>MIPARFAGVLLALALILPGTLCAEGTRGRSSTARCSLFGSDFVNTFDGSMYSFAGYCSYLLAGGCQKRSFSIIGDFQNGKRVSLSVYLGEFFDIHLFVNGTVTQGDQRVSMPYASKGLYLETEAGYYKLSGEAYGFVARIDGSGNFQVLLSDRYFNKTCGLCGNFNIFAEDDFMTQEGTLTSDPYDFANSWALSSGEQWCERASPPSSSCNISSGEMQKGLWEQCQLLKSTSVFARCHPLVDPEPFVALCEKTLCECAGGLECACPALLEYARTCAQEGMVLYGWTDHSACSPVCPAGMEYRQCVSPCARTCQSLHINEMCQERCVDGCSCPEGQLLDEGLCVESTECPCVHSGKRYPPGTSLSRDCNTCICRNSQWICSNEECPGECLVTGQSHFKSFDNRYFTFSGICQYLLARDCQDHSFSIVIETVQCADDRDAVCTRSVTVRLPGLHNSLVKLKHGAGVAMDGQDVQLPLLKGDLRIQHTVTASVRLSYGEDLQMDWDGRGRLLVKLSPVYAGKTCGLCGNYNGNQGDDFLTPSGLAEPRVEDFGNAWKLHGDCQDLQKQHSDPCALNPRMTRFSEEACAVLTSPTFEACHRAVSPLPYLRNCRYDVCSCSDGRECLCGALASYAAACAGRGVRVAWREPGRCELNCPKGQVYLQCGTPCNLTCRSLSYPDEECNEACLEGCFCPPGLYMDERGDCVPKAQCPCYYDGEIFQPEDIFSDHHTMCYCEDGFMHCTMSGVPGSLLPDAVLSSPLSHRSKRSLSCRPPMVKLVCPADNLRAEGLECTKTCQNYDLECMSMGCVSGCLCPPGMVRHENRCVALERCPCFHQGKEYAPGETVKIGCNTCVCRDRKWNCTDHVCDATCSTIGMAHYLTFDGLKYLFPGECQYVLVQDYCGSNPGTFRILVGNKGCSHPSVKCKKRVTILVEGGEIELFDGEVNVKRPMKDETHFEVVESGRYIILLLGKALSVVWDRHLSISVVLKQTYQEKVCGLCGNFDGIQNNDLTSSNLQVEEDPVDFGNSWKVSSQCADTRKVPLDSSPATCHNNIMKQTMVDSSCRILTSDVFQDCNKLVDPEPYLDVCIYDTCSCESIGDCACFCDTIAAYAHVCAQHGKVVTWRTATLCPQSCEERNLRENGYECEWRYNSCA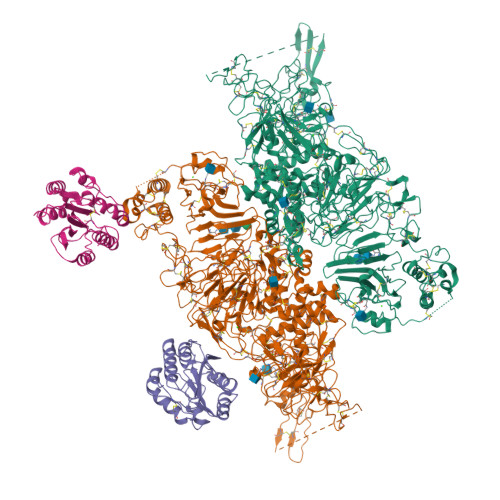PACQVTCQHPEPLACPVQCVEGCHAHCPPGKILDELLQTCVDPEDCP[2x];>PPLHDFYCSRLLDLVFLLDGSSRLSEAEFEVLKAFVVDMMERLRISQKWVRVAVVEYHDGSHAYIGLKDRKRPSELRRIASQVKYAGSQVASTSEVLKYTLFQIFSKIDRPEASRITLLLMASQEPQRMSRNFVRYVQGLKKKKVIVIPVGIGPHANLKQIRLIEKQAPENKAFVLSSVDELEQQRDEIVSYLCDLAPE[2x]> MFERFTDRARRVVVLAQEEARMLNHNYIGTEHILLGLIHEGEGVAAKSLESLGISLEGVRSQVEEIIGQGQQAPSGHIPFTPRAK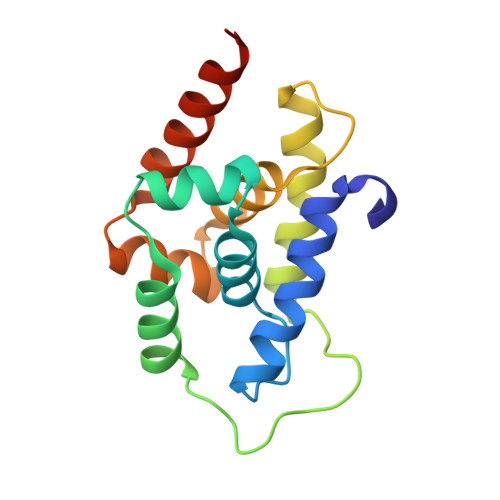KVLELSLREALQLGHNYIGTEHILLGLIREGEGVAAQVLVKLGAELTRVRQQVIQLLSGYLEHHHHHH> MITTPLVHVASVEKGRSYEDFQKVYNAIALKLREDDEYDNYIGYGPVLVRLAWLISGTWDKHDNTGGSYGGTYRFKKEFNDPSNAGLQNGFKFLEPIHKEFPWISSGDLFSLGGVTAVQEMQGPKIPWRCGRVDTPEDTTPDNGRLPDADKDAGYVRTFFQRLNMNDREVVALMGAHALGKTHLKNSGYEGPWGAANNVFTNEFYLNLLNEDWKLEKNDANNEQWDSKSGYMMLPTDYSLIQDPKYLSIVKEYANDQDKFFKDFSKAFEKLLENGITFPKDAPSPFIFKTL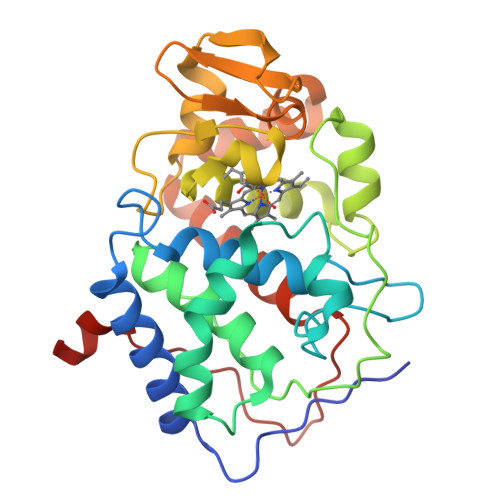EEQGL Fungal degradation of lignin, a key step in carbon recycling in land ecosystems, has been described as an ‘enzymatic combustion’, in which high redox-potential haem peroxidases – the so-called lignin peroxidases (LiPs), manganese peroxidases (MnPs) and versatile peroxidases (VPs) – play a central role. Recent evolutionary studies show that MnPs evolved from fungal generic peroxidases (similar to plant peroxidases) by developing an Mn-binding site formed by three acidic residues near the haem propionates, as shown in the first MnP crystal structure. The genome of Ceriporiopsis subvermispora includes 13 manganese peroxidase (MnP) genes representative of the three subfamilies described in ligninolytic fungi, which share an Mn2+-oxidation site and have varying lengths of the C-terminal tail. We have solved the crystal structure of the extralong MnP6 from C. subvermispora after its heterologous expression.

At the same time, the first crystal structure of an extralong MnP was solved from this fungus and was compared with the known structures of other MnPs. The upper domain is mainly helical with a first structural Ca2+ ion, whereas the lower domain contains α-helices and a non-ordered region stabilized by a second Ca2+ ion. The recombinant MnPs include two structural Ca2+ ions that are incorporated during in vitro folding, but have never been in contact with Mn2+ or Cd2+. The first crystal structure of a short MnP has recently been solved by Fernández-Fueyo et al., and its comparison with the first extralong MnP structure solved here shows a C-tail extension (Gly348–Pro365 in C. subvermispora MnP6) surrounding the entrance of the haem-propionate channel. Such a disposition limits the access of some substrates through this channel, as revealed by diffusion simulations. The tail goes up to near the top of the protein and then turns down towards the region between the Mn2+-binding site (haem-propionate channel) and the main haem-access channel. At the beginning of the tail, the long/extralong MnPs present one extra disulfide bridge that forms a turn pointing towards the surface. The last two differences result in a protrusion below the Mn2+-binding site that causes some access restrictions in long and extralong MnPs. 50 was observed, revealing that the presence of the tail does not always result in decreased MnP stability. This is explained by the numerous interactions with the protein body observed in the extralong MnP crystal structure, including three hydrophobic/hydrophilic patches. The tail, which is anchored by numerous contacts, not only affects the catalytic properties of long/extralong MnPs but is also associated with their high acidic stability.

> MAPTAVCSDGTRVSNAVCCDFVSLGQDLQSMVLQGDCGEDAHEIIRLTFHDAVAISRKLGPSAGGGADGSMLLFPLVEPEFAASNGIDDSVNNLIPFLSLHPTISAGDLVQFAGAVALSNCPGAPRVQFLAGRPNHTIAAIDGLIPEPQDNVTSILERFDDAGGFTPFEVVSLLASHTIARADKVDPTLDAAPFDTTPFTFDSQIFLEVLLKGVGFPGLDNNTGEVSSPLPLGDTSTGGKDTGLMRLQSDFALAHDPRTACFWQGFVDQQEFMSQSFASAFAKLAVLGHNTDDLIDCSEVVPVPKPAVDKPTTFPATTGPQDLELSCLAERFPTLSVDPGAQETLIPHCSDGLENCTSVQFSGPATDSP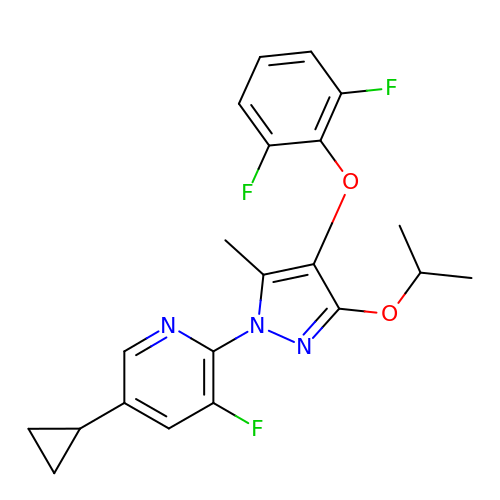2-[4-[2,6-bis(fluoranyl)phenoxy]-5-methyl-3-propan-2-yloxy-pyrazol-1-yl]-5-cyclopropyl-3-fluoranyl-pyridine | C21 H20 F3 N3 O2 | JNAABFZPXJJMPX-UHFFFAOYSA-N> MKLTIWCSEKQVDILQKLGEEFKAKYGIPVEVQYVDFGSIKSKFLTAAPQGQGADIIVGAHDWVGELAVNGLIEPIPNFSDLKNFYDTALKAFSYGGKLYGVPYAMEAVALIYNKDYVDSVPKTMDELIEKAKQIDEEYGGEVRGFIYDVANFYFSAPFILGYGGYVFKETPQGLDVTDIGLANEGAVKGAKLIKRMIDEGVLTPGDNYGTMDSMFKEGLAAMIINGLWAIKSYKDAGINYGVAPIPELEPGVPAKPFVGVQGFMINAKSPNKVIAMEFLTNFIARKETMY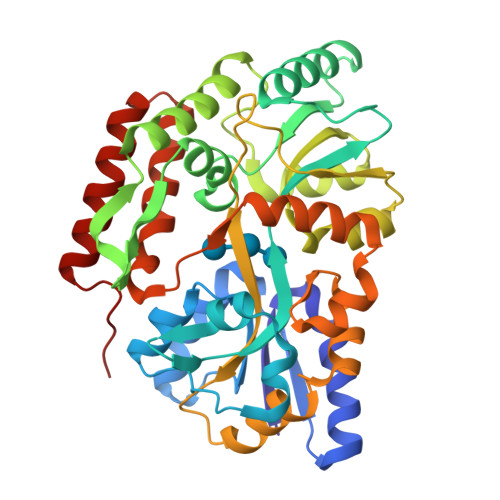KIYLADPRLPARKDVLELVKDNPDVVAFTQSASMGTPMPNVPEMAPVWSAMGDALSIIINGQASVEDALKEAVEKIKAQIEKGSHHHHHH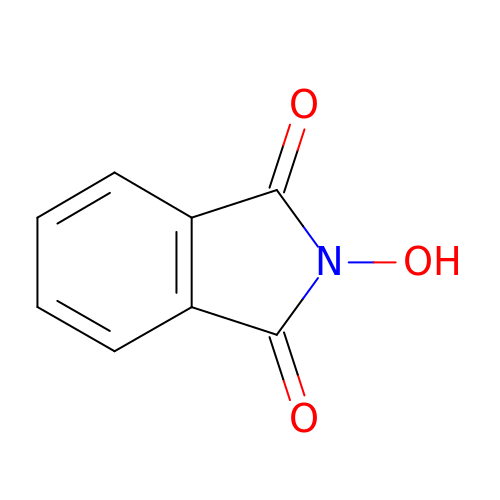2-oxidanylisoindole-1,3-dione | C8 H5 N O3 | CFMZSMGAMPBRBE-UHFFFAOYSA-N>[72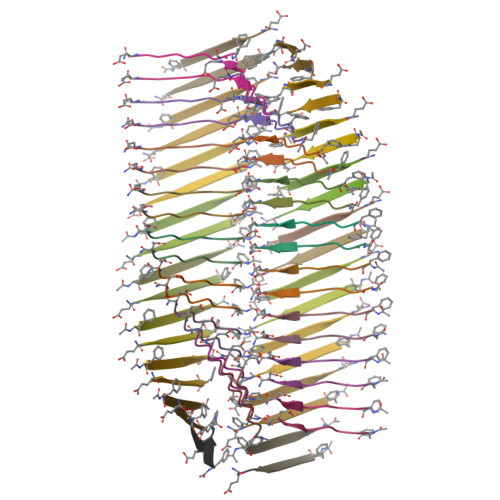x]FKFEFKFE>[12x]GSHMAKYTKEDIFRFADEQNVKFIRLQFTDILGIIKNVEIPVSQLKKALDNKIMFDGSSIEGFVRIEESDMYLFPDLDTWVVFPWTAEKGKVARMICDIYNPDMTPFAGDPRANLKRVLKEMEELGFTEFNLGPEPEFFLFKLDENRRPTLELNDSGGYFDLAPTDLGENCRRDIVLELEEMGFEIEASHHEVAPGQHEIDFKYEDAITACDSIQTFKLVVKTIARKHGLHATFMPKPLFGVNGSGMHFNMSLFNEKGNAFFDESGELELSQTAYHFLAGMLKHARGYTAVTNPTINSFKRLVPGYEAPCYIAWSGKNRSPLVRVPSSRGLSTRLELRSVDPSANPYLAMAVLLKAGLSGIKDELTPPAPVDRNIYGMNEEEREATGIYDLPESLGHALIELEKNEIIKDGLGEHIFEHFIEAKTIECDMFRTAVHPWEREQYLEIY

In Gram-positive bacteria, nitrogen homeostasis is controlled by an operon encoding glutamine synthetase (GS), a dodecameric machine that assimilates ammonium into glutamine, and the GlnR repressor. GlnR detects nitrogen excess indirectly by binding glutamine-feedback-inhibited-GS (FBI-GS), which activates its transcription-repression function. GS generates glutamine from glutamate, ATP, and ammonium by a mechanism that involves the initial phosphorylation of the γ-carboxyl group of glutamate by ATP and the subsequent incorporation of ammonium. The structures show FBI-GS binds the GlnR C-terminal domain within its active-site cavity, juxtaposing two GlnR monomers to form a DNA-binding-competent GlnR dimer.

To visualize the active, transition state (TS) conformations of the GS proteins we reacted them with l-methionine-S-sulfoximine (MSO) in the presence of ATP and solved the structures. In these structures, the Met-Sox-P methyl group occupies the ammonium substrate binding site, thus mimicking the GS transition state and preventing further reaction. Structures of the Pp, Lm, and Sa GS-Met-Sox-P-ADP complexes were obtained to 1.98, 3.50, and 2.95 Å resolution, respectively. These structures were all dodecameric and densities for Met-Sox-P and ADP were clearly observed in each enzyme. The GS TS structures all display the same contacts to the Met-Sox-P and ADP. The resultant ammonia would then be in an ideal position to attack the γ-glutamyl phosphate intermediate. Thus, the GSI-α·Met-Sox-P·ADP complexes mimic the tetrahedral adduct, formed before the generation of the glutamine and inorganic phosphate products. Strikingly, while the TS structures are similar to each other, they show significant differences, both global and local, when compared to the corresponding apo and FBI-GS-GlnR bound states (as apo and FBI-GS-GlnR conformations are the same, the state will be referred to as apo/FBI-GS-GlnR). Although all GS active site loops are altered upon TS formation, residues in the D50´ loop undergo the most dramatic structural rearrangements. In the TS state, Asp62´ and Arg316 are repositioned to provide an optimal active site architecture. Thus, our structural analyses indicate that GS enzymes from low G + C Gram-positive bacteria adopt two distinct states, the active, TS conformation (herein termed the “A” state) and the conformation adopted by apo GS/FBI-GS-GlnR, termed the “I” or inhibited state.> SEFKVTVCFGRTRVVVPCGDGRMKVFSLIQQAVTRYRKA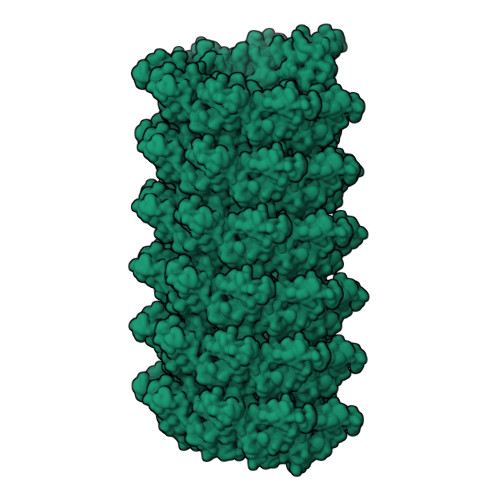VAKDPNYWIQVHRLEHGDGGILDLDDILCDVADDKDRLVAVFDEQ>[2x]ANPLYQKHIISINDLSRDDLNLVLATAAKLKANPQPELLKHKVIASCFFEASTRTRLSFQTSMHRLGASVVGFSDSANTSLGKKGETLADTISVISTYVDAIVMRHPQEGAARLATEFSGNVPVLNAGDGSNQHPTQTLLDLFTIQQTEGRLDNLHVAMVGDLKYGRTVHSLTQALAKFDGNRFYFIAP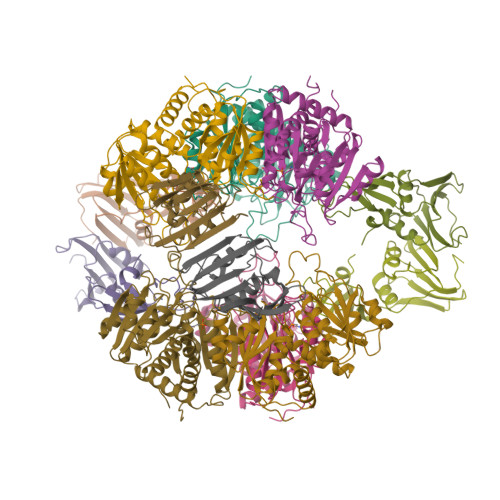DALAMPEYILDMLDEKGIAWSLHSSIEEVMAEVDILYMTRVQKERLDPSEYANVKAQFVLRASDLHNAKANMKVLHPLPRVDEIATDVDKTPHAWYFQQAGNGIFARQALLALVLNRDLVL;>MTHDNKLGVEAIKRGTVIDHIPAQIGFKLLSLFKLTETDQRITIGLNLPSGEMGRKDLIKIENTFLSEDQVDQLALYAPQATVNRIDNYEVVGKSRPSLPERIDNVLVCPNSNCISHAEPVSSSFAVRKRANDIALKCKYCEKEFSHNVVLAN[2x]>MISHSELRKLFYSADAVCFDVDSTVIREEGIDELAKICGVEDAVSEMTRRAMGGAVPFKAALTERLALIQPSREQVQRLIAEQPPHLTPGIRELVSRLQERNVQVFLISGGFRSIVEHVASKLNIPATNVFANRLKFYFNGEYAGFDETQPTAESGGKGKVIKLLKE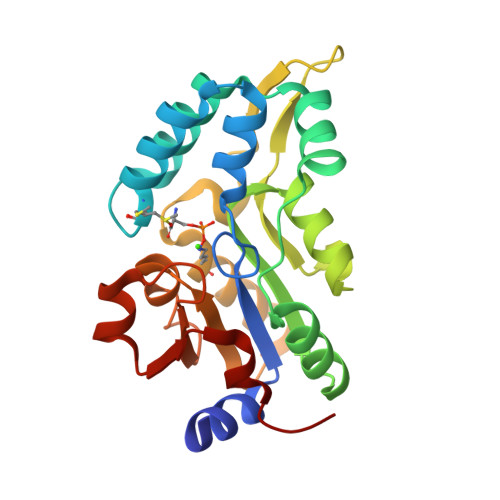KFHFKKIIMIGDGATDMEACPPADAFIGFGGNVIRQQVKDNAKWYITDFVELLGELE[2x]By contrast, in vertebrates the clustered protocadherins (Pcdhs) provide analogous cell-surface diversity, but in this case generated through stochastic alternative promoter choice. Biophysical measurements with domain-deleted proteins showed that Pcdhs also interact in cis, through a membrane-proximal dimer interface involving extracellular cadherin domain 6 (EC6) and potentially EC5. The specificity-determining cell-cell recognition interface of Pcdhs involves domains EC1–4, as shown experimentally through mutagenesis analysis and suggested by mutation correlation analysis.

From these experiments we obtained crystals of γA4EC3–6 and γB2EC3–6, which diffracted to sufficient resolution for crystal structure determination. X-ray diffraction by the γA4EC3–6 crystals was significantly anisotropic, and therefore anisotropic resolution limits were applied. The resolution of the final refined structures was 3.0/4.3/2.85 Å for γA4EC3–6 and 2.3 Å for γB2EC3–6. The two structures are similar overall (RMSD of 3.02 Å over 405 Cα’s), although γA4EC3–6 shows a more pronounced EC4–EC5 bend angle (32.6° for γA4 vs. 18.6° for γB2). These are the first Pcdh structures containing EC6, which displays the classic beta sandwich fold, but with a large insertion between the A and A’ strands. Notably the G-strands of both EC6 domains are decorated with O-mannose groups on neighboring surface-facing residues, three for γB2 and four for γA4. The γA4EC3–6 structure did not show any protein:protein interactions consistent with cis interactions in the crystal which, given that this γA family member is monomeric in solution, was expected. Furthermore, O-mannosylation is observed at EC6 G-strand residues 624, 626, and 628 (γB2 numbering) of both the γB2 and γA4 structures—on the opposite molecular face to the mutations that disrupt cell surface delivery.

> NAPVFTQPEYHISVKENLPVGTRLLTIKATDPDEGVNGEVTYSFRNVREKISQLFQLNSLTGDITVLGELDYEDSGFYDVDVEAHDGPGLRARSKVLVTVLDVNDNAPEVTVTSLTSSIQEASSPGTVIALFNVHDSDSGENGLVTCSIPDNLPFRLEKTYGNYHRLLIHRTLDREEVSDYNITITATDQGTPPLSTETYISLQVVDINDNPPTFTHASYSAYIPENNPRGASILSITAQDPDSGENAQVIYSLSEDTIQGAPMSSYVSINSNTGVLYALRSFDYEQFQDLKLLVTARDSGTPPLSSNVSLSLSVLDQNDNTPEILYPTIPTDGSTGVELTPRSADPGYLVTKVVAVDKDSGQNAWLSYRLLKASEPGLFSVGLHTGEVRTARALLDRDALKQSLVVTVQDHGQPPLSATVTLTIAVSDNIPDHHHHHHHH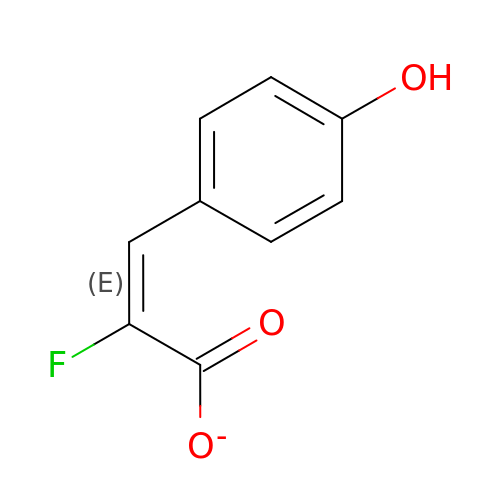2-FLUORO-3-(4-HYDROXYPHENYL)-2E-PROPENEOATE | C9 H6 F O3 | SBIZDOWXYPNTOJ-VMPITWQZSA-M>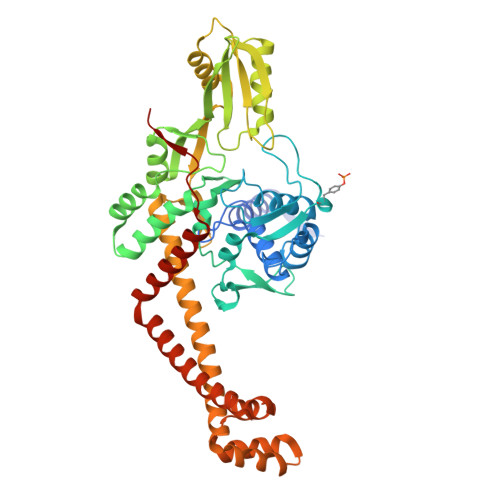 TDTTLPPDDSLDRIEPVDIEQEMQRSYIDYAMSVIVGRALPEVRDGLKPVHRRVLYAMFDSGFRPDRSHAKSARSVAETMGNYHPHGDASIYDSLVRMAQPWSLRYPLVDGQGNFGSPGNDPPAAMRYTEARLTPLAMEMLREIDEETVDFIPNYDGRVQEPTVLPSRFPNLLANGSGGIAVGMATNIPPHNLRELADAVFWALENHDADEEETLAAVMGRVKGPDFPTAGLIVGSQGTADAYKTGRGSIRMRGVVEVEEDSRGRTSLVITELPYQVNHDNFITSIAEQVRDGKLAGISNIEDQSSDRVGLRIVIEIKRDAVAKVVINNLYKHTQLQTSFGANMLAIVDGVPRTLRLDQLIRYYVDHQLDVIVRRTTYRLRKANERAHILRGLVKALDALDEVIALIRASETVDIARAGLIELLDIDEIQAQAILDMQLRRLAALERQRIIDDLAKIEAEIADLEDILAKPERQRGIVRDELAEIVDRHGDDRRTRIIAIGSG> MERNKLARQIIDTCLEMTRLGLNQGTAGNVSVRYQDGMLITPTGIPYEKLTESHIVFIDGNGKHEEGKLPSSEWRFHMAAYQSRPDANAVVHNHAVHCTAVSILNRSIPAIHFMIAAAGGNSIPCAPYATFGTRELSEHVALALKNR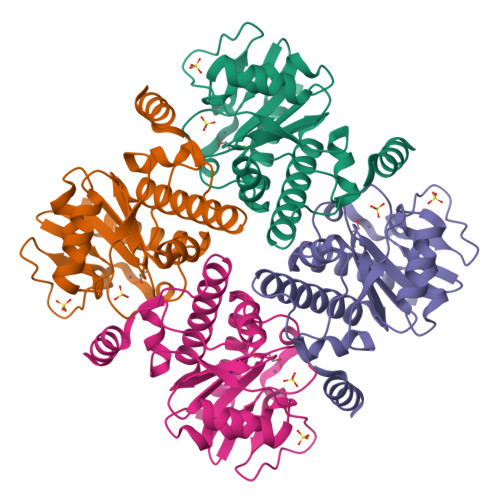KATLLQHHGLIACEVNLEKALWLAHEVEVLAQLYLTTLAITDPVPVLSDEEIAVVLEKFKTYGLRIEE>[2x]SMSSSGDKEVIAKTDAGDVTKGELYTNMKKTAGASVLTQLVQEKVLDKKYKVSDKEIDNKLKEYKTQLGDQYTALEKQYGKDYLKEQVKYELLTQKAAKDNIKVTDADIKEYWEGLKGKIRASHILVADKKTAEEVEKKLKKGEKFEDLAKEYSTDSSASKGGDLGWFAKEGQMDETFSKAAFKLKTGEVSDPVKTQYGYHIIKKTEERGKYDDMKKELKSEVLEQKLNDNAAVQEA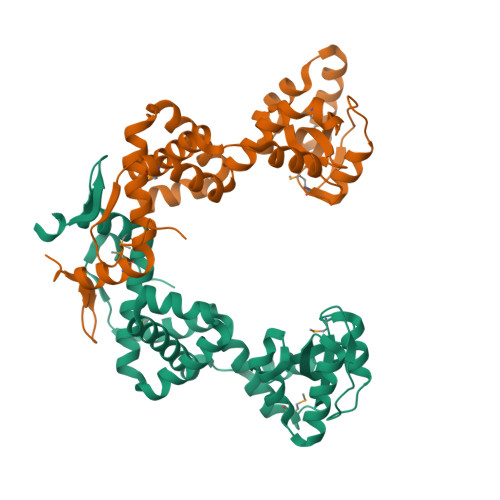VQKVMKKADIEVKDKDLKDTFNTSST> QSMLRAQATGNIGVLVSRVTNPFFAGLFDAIERELHAHGYQVMITQTYDDPEAEERFLKQLKSRELDGVILASVEAPDRVMAVAKAFPGRVVVVNADVQIPGATSLVLPHYQATRDALDYLFNQGHRRFAYVSGGTISGAHHGQSRTQAFLDFMQAHQLLVAQDLLFGQIHTAKEGQAVGKQLASLAPNVRPDAVFTNSDEVAVGVIDSLLAADVKVPDDIAVMGYDDQPFAPFAKIPLTTVHQPVASMAAAATHELLKGLGRQVAQDTQPTLHLSLKI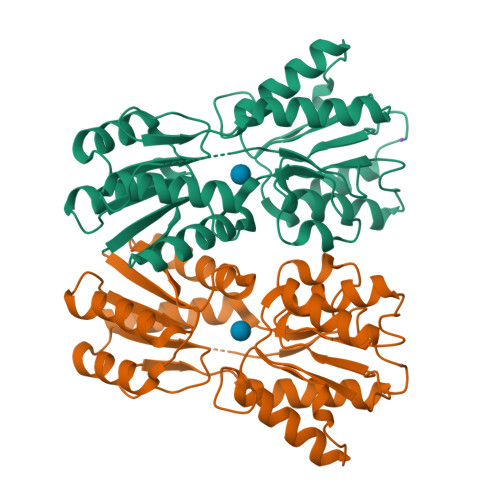RQSA>GSSPSLEQDDGDEETSVVIVGKISFCPKDVLGHGAEGTIVYRGMFDNRDVAVKRILPECFSFADREVQLLRESDEHPNVIRYFCTEKDRQFQYIAIELCAATLQEYVEQKDFAHLGLEPITLLQQTTSGLAHLHSLNIVHRDLKPHNILISMPNAHGKIKAMISDFGLCKKLAVGRHSFSRRSGVPGTEGWIAPEMLSEDCKENPTYTVDIFSAGCVFYYVISEGSHPFGKSLQRQANILLGACSLDCLHPEKHEDVIARELIEKMIAMDPQKRPSAKHVLKHPFFWSLEKQLQFFQDVSDRIEKESLDGPIVKQLERGGRAVVKMDWRENITVPLQTDLRKFRTYKGGSVRDLLRAMRNKKHHYRELPAEVRETLGSLPDDFVCYFTSRFPHLLAHTYRAMELCSHERLFQPYYFHEPPEPQPPVTPDALGNS[2x]

IRE1 integrates multiple functional domains into a single ER-membrane-spanning protein. The lumenal domain senses unfolded proteins in the ER through indirect and direct mechanisms: as a result, it undergoes dimerization and subsequent oligomerization. The association of the lumenal domain promotes dimerization and oligomerization of the cytoplasmic kinase-RNase tandem domain. The cytoplasmic domain has been shown to self-associate via different surface contacts, where a back-to-back (B2B) configuration is believed to fulfill the essential structural requirements for RNase activation.

In the biochemical RNase assay we found that less bulky substituents like buten- or butynamide (compound 1 and G-7658, respectively) led to higher RNase activation, while larger substituents such as branched and longer carbamates or amides (compounds 6-12) led to inhibition. We then co-crystallized a more potent allosteric RNase activator from our SAR effort, G-7658, with IRE1-0P and found that it superimposes perfectly with G-1749, except for an increase of approximately 0.5 Å in distance from E612. More potent allosteric RNase activators of IRE1-0P, such as G-7658, inhibited IRE1-3P only partially, suggesting that perhaps certain compounds experience mixed binding modes in the presence of phosphorylation, where their tail can be accommodated in either the front or back pocket. In an alternative scenario, an upward conformation of the loop in absence of phosphorylation in a B2B dimer can increase activity of the RNase domain. We show in our work that this kind of activation can be brought upon by small molecules such as G-1749 and G-7658, but whether this modulation is physiologically relevant remains to be seen.> VGEEGTGGTVHLLCLAASSGVPLFCRSSRGGAPARQQLPFSVIGSLNGVHMFGQNLEVQLSSARTENTTVVWKSFHDSITLIVLSSEVGISELRLERLLQMVFGAMVLLVGLEELTNIRNVERLKKDLRASYCLIDSFLGDSELIGDLTQCVDCVIPPEGSLLQEALSGFAEAAGTTFVSLVVSGRVVAATEGWWRLGTPEAVLLPWLVGSLPPQTARDYPVYLPHGSPTVPHRLLTLTLLPSLELCLLCGPSPPLSQLYPQLLERWWQPLLDPLRACLPLGPRALPSGFPLHTDILGLLLLHLELKRCLFTVEPLGDKEPSPEQRRRLLRNFYTLVTSTHFPPEPGPPEKTEDEVYQAQLPRACYLVLGTEEPGTGVRLVALQLGLRRLLLLLSPQSPTHGLRSLATHTLHALTPLL;> MDYKDDDDKGVPRIPMASVASCDSRPSSDELPGDPSSQEEDEDYDFEDRVSDSGSYSS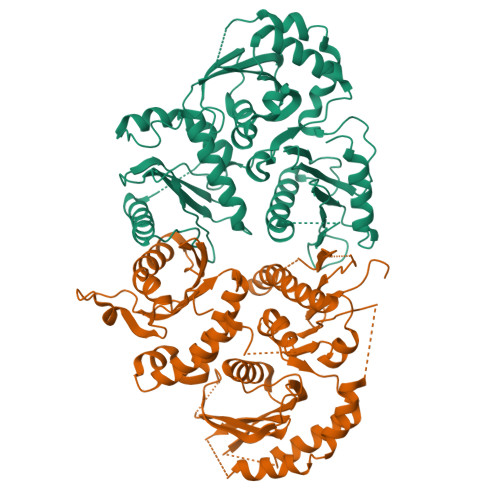ASSDYDDLEPEWLDSVQKNGELFYLELSEDEEESLLPETPTVNHVRFSENEIIIEDDYKERKKYEPKLKQFTKILRRKRLLPKRCNKKNSNDNGPVSILKHQSNQKTGVIVQQRYKDVNVYVNPKKLTVIKAKEQLKLLEVLVGIIHQTKWSWRRTGKQGDGERLVVHGLLPGGSAMKSGQVLIGDVLVAVNDVDVTTENIERVLSCIPGPMQVKLTFENAYDVKRETSHPRQKKTQSNTSDLVKLLWGEEVEGIQQSGLNTPHIIMYLTLQLDSETSKEEQEILYHYPMSEASQKLKSVRGIFLTLCDMLENVTGTQVTSSSLLLNGKQIHVAYWKESDKLLLIGLPAEEVPLPRLRNMIENVIQTLKFMYGSLDSAFCQIENVPRLDHFFNLFFQRALQPAKLHSSASPSAQQYDASSAVLLDNLPGVRWLTLPLEIKMELDMALSDLEAADFAELSEDYYDMRRLYTILGSSLFYKGYLICSHLPKDDLIDIAVYCRHYCLLPLAAKQRIGQLIIWREVFPQHHLRPLADSSTEVFPEPEGRYFLLVVGLKHYMLCVLLEAGGCASKAIGSPGPDCVYVDQVKTTLHQLDGVDSRIDERLASSPVPCLSCADWFLTGSREKTDSLTTSPILSRLQGTSKVATSPTCRRTLFGDYSLKTRKPSPSCSSGGSDNGCEGGEDDGFSPHTTPDAVRKQRESQGSDGLEESGTLLKVTKKKSTLPNPFHLGNLKKDLPEKELEIYNTVKLTSGPENTLFHYVALETVQGIFITPTLEEVAQLSGSIHPQLIKNFHQCCLSIRAVFQQTLVEEKKKGLNSGDHSDSAKSVSSLNPVKEHGVLFECSPGNWTDQKKAPPVMAYWVVGRLFLHPKPQELYVCFHDSVTEIAIEIAFKLFFGLTL> SNVQTSADRVPHDLSHLVFEAGKIGRLKTISWTPVVAGDSFECDMVGAIRLSPLRRGLAVDSRVDIFSFYIPHRHIYGQQWINFMKDGVNASPLPPVTCSSGWDSAAYLGTIPSSTLKVPKFLHQGYLNIYNNYFKPPWSDDLTYANPSNMPSEDYKWGVRVANLKSIWTAPLPPDTRTSENMTTGTSTIDIMGLQAAYAKLHTEQERDYFMTRYRDIMKEFGGHTSYDGDNRPLLLMRSEFWASGYDVDGTDQSSLGQFSGRVQQTFNHKVPRFYVPEHGVIMTLAVTRFPPTHEMEMHYLVGKENLTYTDIACDPALMANLPPREVSLKEFFHSSPDSAKFKIAEGQWYRTQPDRVAFPYNALDGFPFYSALPSTDLKDRVLVNTNNYDEIFQSMQLAHWNMQTKFNINVYRHMPTTRDSIMTS;> MFQKFISKHNAPINSTQLAATKTPAVAAPVLSVPNLSRSTILINATTTAVTTHSGLCHVVRIDETNPTNHHALSIA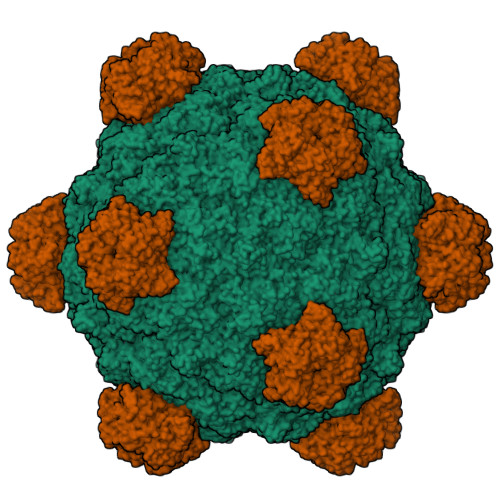GSLSNVPADMIAFAIRFEVADGVVPTAVPALYDVYPIETFNNGKAISFKDAVTIDSHPRTVGNDVYAGIMLWSNAWTASTISGVLSVNQVNREATVLQPLK;> MKKSIRRSGGKSKGARLWYVGGTQY>SVIEFGKMIQEETDKNPLTSYSFYGCHCGLGNGGKPKDATDRCCFVHSCCYASLSDCSPATNRYSYHKEGGAIVCGSSTPCKGQICECDKAAA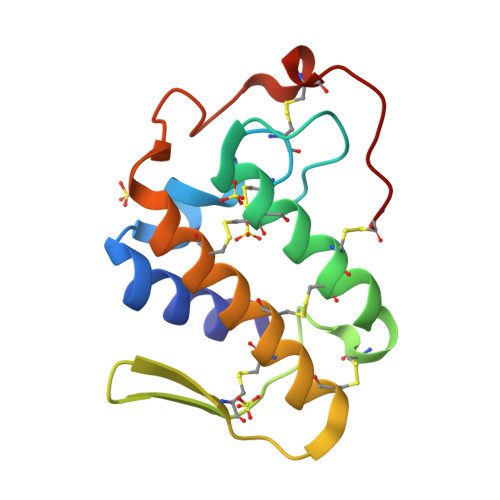ICFKENLKTYNKKYKVYLRFKCKGVSEKC[8x]>QTVTGGLRSLYQRKVLPLEEAYRFHEFHSPALEDADFENKPMILLVGQYSTGKTTFIRYLLEQDFPGMRIGPEPTTDSFIAVMYGETEG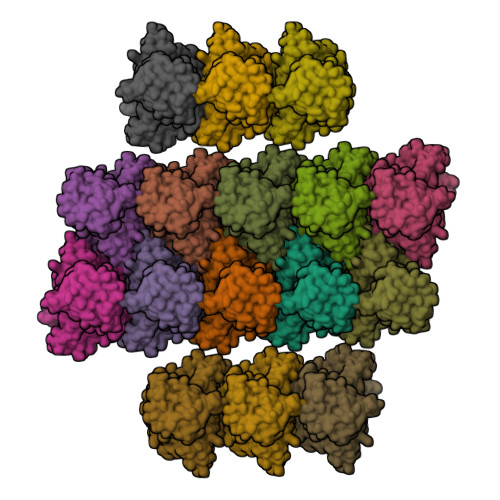STPGNALVVDPKKPFRKLSRFGNAFLNRFMCSQLPNQVLKSISIIDSPGILSGEKQRISRGYDFCQVLQWFAERVDRIILLFDAHKLDISDEFSEAIKAFRGQDDKIRVVLNKADQVDTQQLMRVYGALMWSLGKVINTPEVLRVYIGSFWAQPLQNTDNRRLFEAEAQDLFRDIQSLPQKAAVRKLNDLIKRARLAKVHAYIISYLKKEMPNMFGKENKKRELIYRLPEIYVQLQREYQISAGDFPEVKAMQEQLENYDFTKFHSLKPKLIEAVDNMLTNKISSLMGLISQEEMNMPTQMVQGGAFDGTTEGPFNQGYGEGAKEGADEEEWVVAKDKPVYDELFYTLSPINGKISGVNAKKEMVTSKLPNSVLGKIWKLADCDCDGMLDEEEFALAKHLIKIKLDGYELPNSLPPHLVPPSHRK[16x]>MSYTREDIIRIAEEENVRFIRLQFTDLLGTIKNVEIPVSQLEKALDNKMMFDGSSIEGYVRIEESDMYLYPDLDTWVVFPWVTSDRVARLICDIYKPDGSPFAGDPRGILKRVLKEAEELGYTSMNVGPEPEFFLFKTDEKGDPTTELNDQGGYFDLAPMDLGENCRREIVLKLEEMGFEIEASHHEVAPGQHEIDFKYADAVKAADQIQTFKLVVKTIARQHGLHATFMPKPLFGVNGSGMHCNQSLFKDNENVFYDETDELGLSQTARHYMAGILKHARAMAAITNPTVNSYKRLVPGYEAPCYVAWS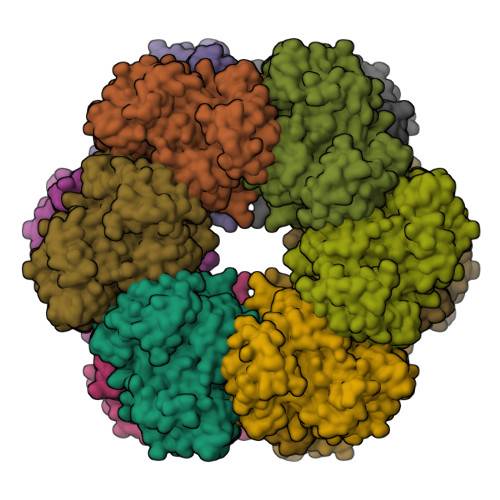ASNRSPMIRIPASRGLSTRVEVRNPDPAANPYLALAVMLRAGLDGIKRQMALPAPIDRNIYVMSEEERIEEGIPSLPADLKEALSELIRSEVISDALGDHALAYFYELKEIEWDMYRTQVHQWERDQYLTLY[3x]>[2x]MNKGELVDAVAEKASVTKK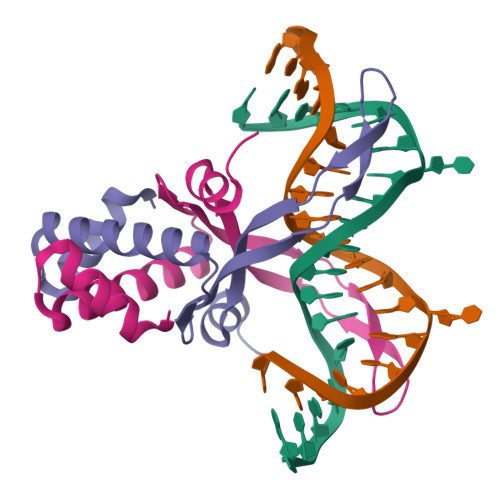QADAVLTAALETIIEAVSSGDKVTLVGFGSFESRERKAREGRNPKTNEKMEIPATRVPAFSAGKLFREKVAPPKA>[2x]MRTQWPSPAKLNLFLYITGQRADGYHTLQTLFQFLDYGDTISIELRDDGDIRLLT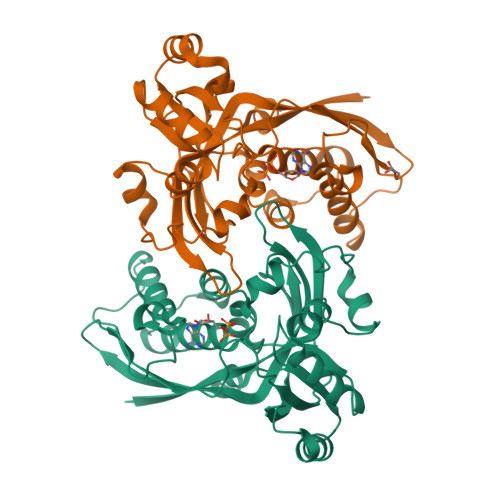PVEGVEHEDNLIVRAARLLMKTAADSGRLPTGSGANISIDKRLPMGGGLGGGSSNAATVLVALNHLWQCGLSMDELAEMGLTLGADVPVFVRGHAAFAEGVGEILTPVDPPEKWYLVAHPGVSIPTPVIFKDPELPRNTPKRSIETLLKCEFSNDCEVIARKRFREVDAVLSWLLEYAPSRLTGTGACVFAEFDTESEARQVLEQAPEWLNGFVAKGVNLSPLHRAML>[4x]MKKILIVSFLGKGRYYETFYYSIEHSEKMVKKRLSPLANAILEKENGNDVEIIFFVTNEVKNEFLYDENNEYAKNILNELNEIKNYGIKVSYRDIPKGKNYEELEIIMEEIEKLLLDFKGNKVIF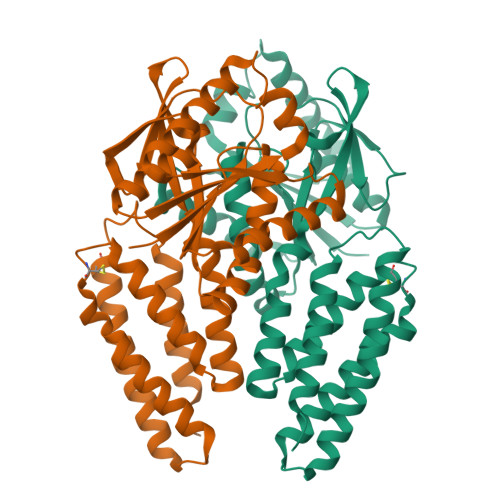DLTHGLRHMAIFTSSTVFYFKNLMEKANKLEMKIVYGAYEIGEEIEKNLKKVPILDITQTLELSDLTIALEEFERYGITERMIIVLKNIQKIVAKNKLCNLNELKFSSLSRELKLFEELLKIPSPPEKIANSIYKINDILESSIREFKLCSKNSENLFFIKPIQKFLVDFQKIVLEKLPLDKKINKYSNIATLEKVEFMKNIIKLLINWKMYSEAVIHLRELLIDIKLIENGKYFYYNNKDFREKYWMYSYNIVDTKDKELPKKIEELLKNVKGWRNSVAHGGRANTSINQKTLEENLENALSMIDEILLSMKDLKVNS2-({N-[(2S)-2,4-dihydroxy-3,3-dimethylbutanoyl]-beta-alanyl}amino)ethyl fluoroacetate | C13 H23 F N2 O6 | 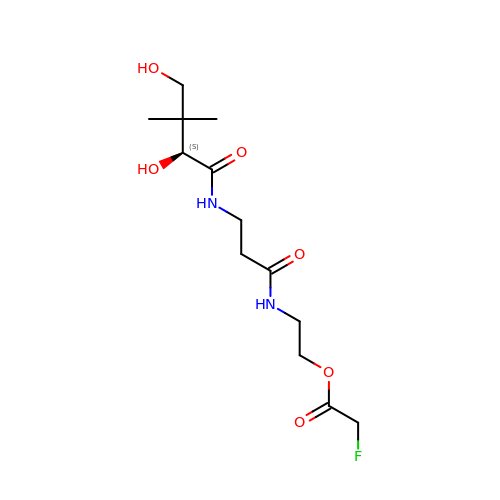ONWRIDRSVIZQIL-LLVKDONJSA-N> APDTSVSNKQNFSTDVIYQIFTDRFSDGNPANNPTGAAFDGTCTNLRLYCGGDWQGIINKINDGYLTGMGVTAIWISQPVENIYSIINDSGVNNTAYHGYWARDFKKTNPAYGTIADFQNLIAAAHAKNIKVIIDFAPNHTSPASPDQPSFAENGRLYDNGTLLGGYTNDTQNLFHHNGGTDFSTTENGIYKNLYDLADLNHNNSTVDVYLKDAIKMWLDLGIDGIRMDAVKHMPFGWQKSFMAAVNNYKPVFTFGEWFLGVNEVSPENHKFANESGMSLLDFRFAQKVRQVFRDNTDNMYGLKAMLEGSAADYAQVDDQVTFIDNHDMERFHASNANRRKLEQALAFTLTSRGVPAIYYGTEQYMSGGTDPDNRARIPSFSTSTTAYQVIQKLAPLRKCNPAIAYGSTQERWINNDVLIYERKFGSNVAVVAVNRNLNAPASISGLVTSLPQGSYNDVLGGLLNGNTLSVGSGGAASNFTLAAGGTAVWQYTAATATPTIGHVGPMMAKPGVTITIDGRGFGSSKGTVYFGTTAVSGADITSWEDTQIKVKIPAVAGGNYNIKVANAAGTASNVYDNFEVLSGDQVSVRFVVNNATTALGQNVYLTGSVSELGNWDPAK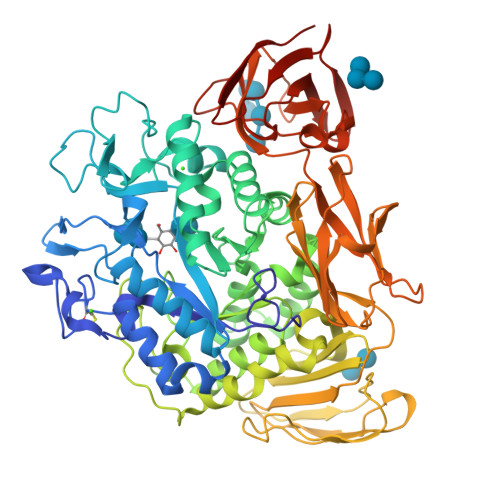AIGPMYNQVVYQYPNWYYDVSVPAGKTIEFKFLKKQGSTVTWEGGSNHTFTAPSSGTATINVNWQP>TRDQNGTWEMESNENFEGYMKALDIDFCTRKIAVR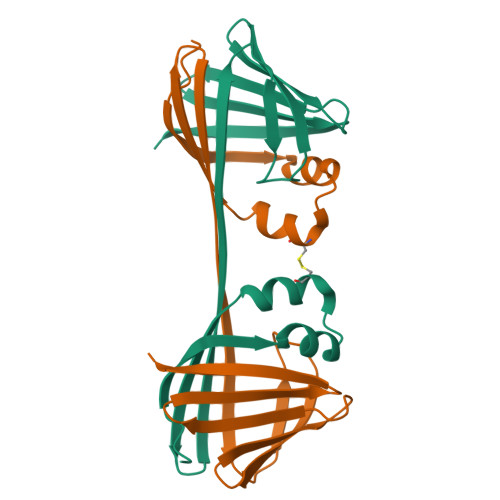CTQTKVIDQDGDNFKDKTTSTFRHHHNYDVDFTVGVEFDEYTKSLDNRHVKALVTWEGDVLVCVQKGEKENRGWKKWIEGDKLYLELTCGDQVCRQVFKKK[2x]>[2x]MEEQIVPFYGKHQAGITTAHQTYVYFAALDVTAKEKSDIITLFRNWTSLTQMLTSGKKMSAEQRNQYLPPQDTGESADLSPSNLTVTFGFGPSFFEKDGKDRFGLKSKKPKHLAALPAMPNDNLDEKQGGGDICIQVCADDEQVAFHALRNLLNQAVGTCEVRFVNKGFLSGGKNGETPRNLFGFKDGTGNQSTEDDSLMNSIV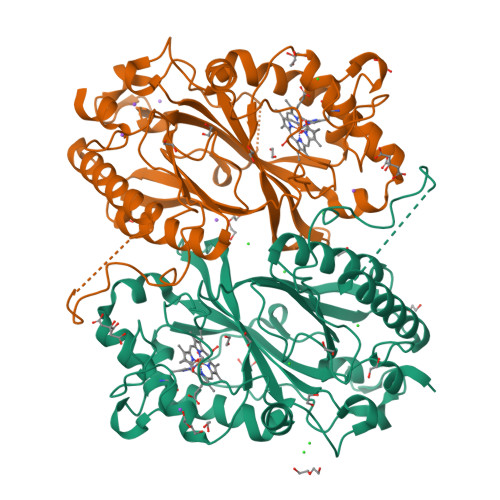WVQSGEPDWMTGGTYMAFRKIKMFLEIWDRSSLKDQEDTFGRRKSSGAPFGQKKETDPVKLNQIPSNSHVSLAKSTGKQILRRAFSYTEGLDPKTGYMDAGLLFISFQKNPDNQFIPMLKALSAKDALNEYTQTIGSALYACPGGCKKGEYIAQRLLES>[2x]MFIKNDHAGDRKRLEDWRIKGYDPLTPPDLLQHEFPISAKGEENIIKARDSVCDILNGKDDRLVIVIGPCSLHDPKAAYDYADRLAKISEKLSKDLLIIMRAYLEKPRTTVGWKGLINDPDMNNSFQINKGLRISREMFIKLVEKLPIAGEMLD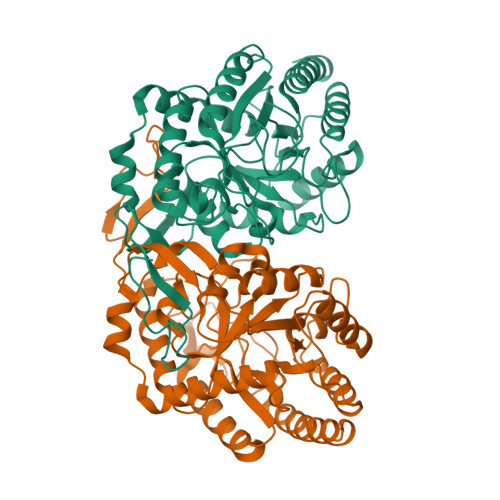TISPQFLSDCFSLGAIGARTTESQLHRELASGLSFPIGFKNGTDGGLQVAIDAMRAAAHEHYFLSVTKPGVTAIVGTEGNKDTFLILRGGKNGTNFDKESVQNTKKQLEKAGLTDDSQKRIMIDCSHGNSNKDFKNQPKVAKCIYDQLTEGENSLCGVMIESNINEGRQDIPKEGGREGLKYGCSVTDACIGWESTEQVLELLAEGVRNRRKALKK>GPGMAVKHLIVLKFKDEITEAQKEEFFKTYVNLVNIIPAMKDVYWGKDVTQKNKEEGYTHIMEVTFESVETIQDYIIHPAHVGFGDVYRSFWEKLLIFDYT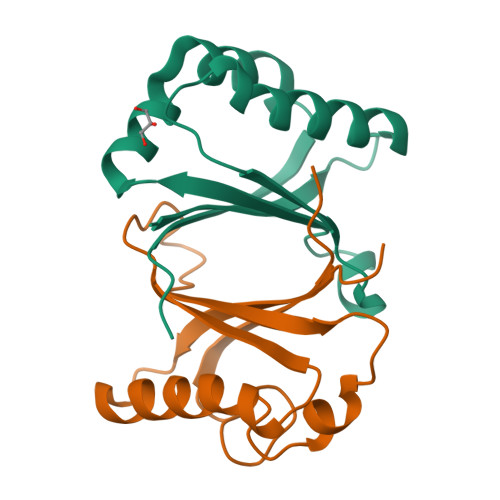PRK[2x]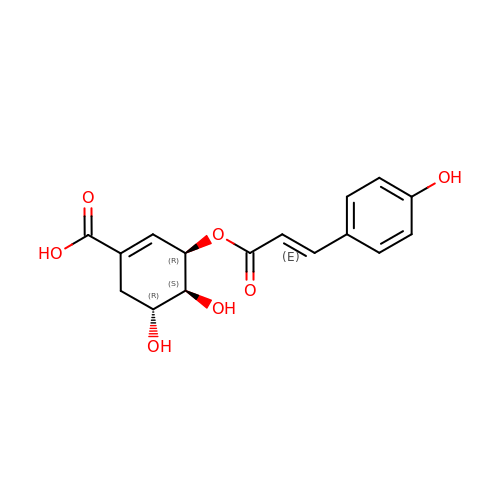(3~{R},4~{S},5~{R})-3-[(~{E})-3-(4-hydroxyphenyl)prop-2-enoyl]oxy-4,5-bis(oxidanyl)cyclohexene-1-carboxylic acid | C16 H16 O7 | LKLFKFQUYFROPV-ADMZAUMBSA-N>[2x]AQWVPR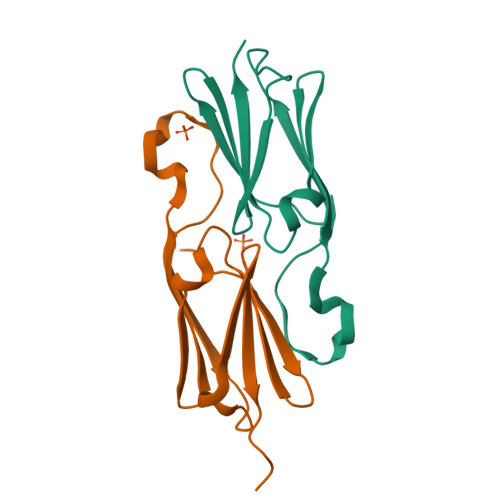VDIKEEVNHFVLYADLPGIDPSQIEVQMDKGILSIRGERKSESSTETERFSRIERRYGSFHRRFALPDSADADGITAAGRNGVLEIRIPKRPAA(1S)-1-CYCLOPROPYL-2-[(2S)-4-(2,5-DIFLUOROPHENYL)-2-PHENYL-2,5-DIHYDRO-1H-PYRROL-1-YL]-2-OXOETHANAMINE 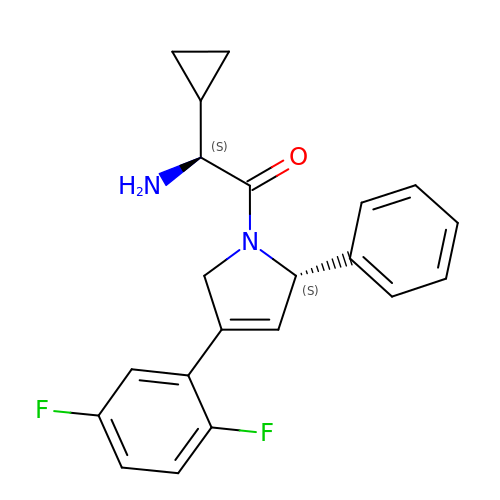| C21 H20 F2 N2 O | VCOUEHUEFUDZIS-PMACEKPBSA-N>MGEFVTPLLETVSSFRPNEFESKFLPPENKPLETALLKRAKELFTNN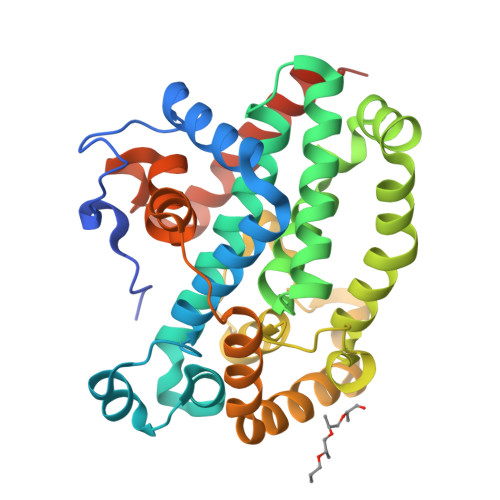DPKVIAQHVLSMDCRVARILGVSEEMRRNMGVSSGLELITLPHGHQLRLDIIERHNTMAIGIAVDILGCTGTLEDRAATLSKIIQVAVELKDSMGDLYSFSALMKALEMPQITRLEKTWTALRHQYTQTAILYEKQLKPFSKLLHEGRESTCVPPNNVSVPLLMPLVTLMERQAVTFEGTDMWEKNDQSCEIMLNHLATARFMAEAADSYRMNAERILAGFQPDEEMNEICKTEFQMRLLWGSKGAQVNQTERYEKFNQILTALSRKLEPPPVKQAELLEHHHHHH[4x]>[2x]MAHHHHHHMPRFAANLSTMFNEVPFLERFRLAAEAGFGGVEFLFPYDFDADVIARELKQHNLTQVLFNMPPGDWAAGERGMAAISGREQEFRDNVDIALHYALALDCRTLHAMSGITEGLDRKACEETFIENFRYAADKLAPHGITVLVEPLNTRNMPGYFIVHQLEAVGLVKRVNRPNVAVQLDLYHAQIMDGDLTRLIEKMNGAFSHV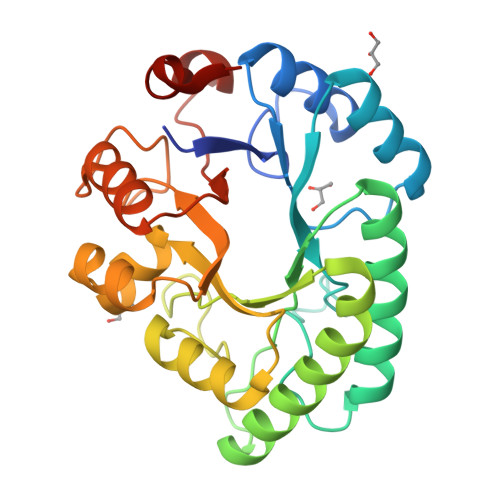QIASVPDRHEPDEGELNYPYLFSVLESVGYRGWVGCEYNPRGKTESGLAWFAPYRDQSA>MECLRSLPCLLPRAMRLPRRTLCALALDVTSVGPPVAACGRRANLIGRSRAAQLCGPDRLRVAGEVHRFRTSDVSQATLASVAPVFTVTKFDKQGNVTSFERKKTELYQELGLQARDLRFQHVMSITVRNNRIIMRMEYLKAVITPECLLILDYRNLNLEQWLFRELPSQLSGEGQLVTYPLPFEFRAIEALLQYWINTLQGKLSILQPLILETLDALVDPKHSSVDRSKLHILLQNGKSLSELETDIKIFKESILEILDEEELLEELCVSKWSDPQVFEKSSAGIDHAEEMELLLENYYRLADDLSNAARELRVLIDDSQSIIFINLDSHRNVMMRLNLQLTMGTFSLSLFGLMGVAFGMNLESSLEEDHRIFWLITGIMFMGSGLIWRRLLSFLGRQLEAPLPPMMASLPKKTLLADRSMELKNSLRLDGLGSGRSILTNRSADYKDDDDK[5x]

Eukaryotic mitochondrial RNA splicing 2 (Mrs2), a homolog of prokaryotic CorA, anchors to the inner mitochondrial membrane and mediates the influx of Mg2+ into the mitochondrial matrix. The overall structure of the hMrs2 channel has a cone shape, and it is assembled into a pentamer with a central pore in the middle. The pentameric hMrs2 structure can be further separated into two parts: the N-terminal funnel domain within the matrix and the C-terminal transmembrane domain in the inner mitochondrial membrane. Molecular dynamics simulations and mitochondrial Mg2+ uptake assays show that the R-ring may function as a charge repulsion barrier, and Cl− may function as a ferry to jointly gate Mg2+ permeation in hMrs2.

The hMrs2 structure was reconstructed from the dataset in the presence of 20 mM Mg2+, pH 8.0 (hereinafter referred to as hMrs2-Mg); from the dataset without the addition of external Mg2+ or EDTA, pH 8.0 (named hMrs2-rest); from the dataset in the presence of 1 mM EDTA, pH 8.0 (named hMrs2-lowEDTA); or from the dataset in the presence of 5 mM EDTA, pH 6.8 (named hMrs2-highEDTA). The final 3D reconstructions of hMrs2-Mg, hMrs2-rest, hMrs2-lowEDTA and hMrs2-highEDTA were determined at overall resolutions of 2.6 Å, 2.9 Å, 2.5 Å and 2.7 Å, respectively. The overall structures of hMrs2-rest, hMrs2-lowEDTA and hMrs2-highEDTA were very similar to that of hMrs2-Mg. Of the five ligand-binding sites, three sites (Mg-1, Mg-2 and Cl-1) but not the other two binding sites (Mg-3 and Mg-4) are located in the three other aforementioned hMrs2 structures (hMrs2-rest, hMrs2-lowEDTA and hMrs2-highEDTA). However, at different pH values and after EDTA treatments at different concentrations, all four hMrs2 structures formed symmetric holo-pentamers. Moreover, the four hMrs2 structures were very similar in terms of the pentamer and protomer structures.>[2x]ASLTEIEHLVQSVCKSYRETCQLRLEDLLRQRSNIFSREEVTGYQRKSMWEMWERCAHHLTEAIQYVVEFAKRLSGFMELCQN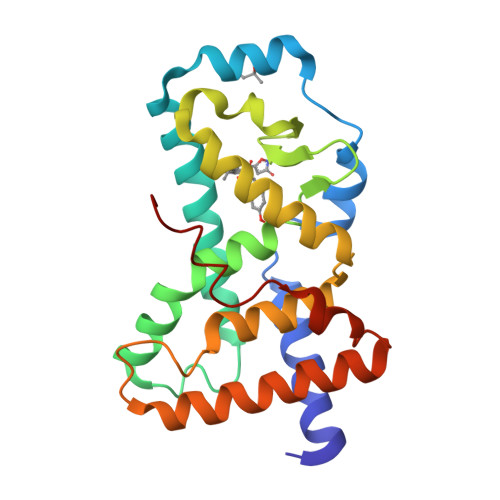DQIVLLKAGAMEVVLVRMCRAYNADNRTVFFEGKYGGMELFRALGCSELISSIFDFSHSLSALHFSEDEIALYTALVLINAHRPGLQEKRKVEQLQYNLELAFHHHLCKTHRQSILAKLPPKGKLRSLCSQH> PTKKVLDENGQSINGKSVLPNATLDYVAKQNFSQYKGIKASAEAIAKGFAFVDQPNEALAELTVKSIKASNGDDVSSLLEMRHVLSKDTLDQKLQSLIKEAGISPVGEFYMWTAKDPQAFYKAYVQKGLDITYNLSFKVKKEFTKGQIKNGVAQIDFGNGYTGNIVVNDLTTPEVHKDVLDKEDGKSIN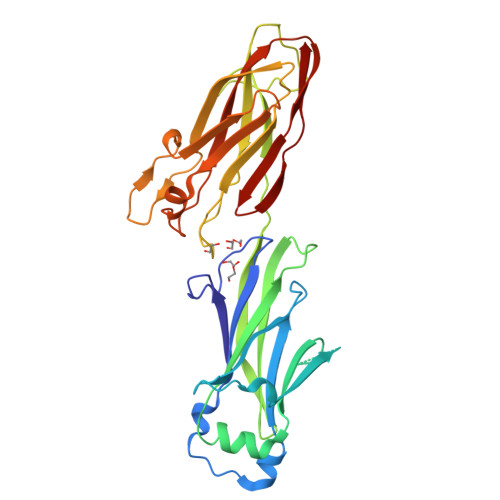NGTVKLGDEVTYKLEGWVVPANRGYDLFEYKFVDHLQHTHDLYLKDKVVAKVAITLKDGTVIPKGTNLVQYTETVYNKETGRYELAFKADFLAQVSRSSAFGADDFIVVKRIKAGDVYNTADFFVNGNKVKTETVVTHT>[4x]SAVKTNVGPSRAGVGYDVIVIGGGFAGVTAAREASRSGLKTLILEGRSRLGGRTFTSKLQNQKVELGGTWVHWTQPNVWTEIMHYGLEVEETVGLANPETVIWVTEDNVKRAPAAEAFEIFGSACNEYYKEARNIYPRPFEPFFERKKLQHVDGLSAADY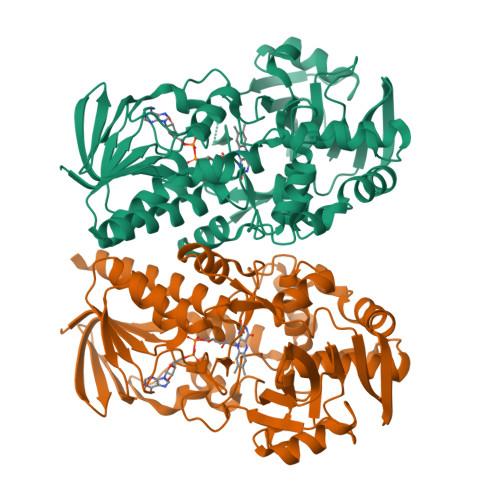LEKLPLTREQKDMMDSWLSGNGHNYPETIAYSEIMRWFALSNFNMPTMFDSIARYKIKTGTHSLLEAIMADGNSEVKLSTPVTKVNQDKDKVTVTTEDGVFTASAVIVAVPINTLHDIEYSPKLSAAKVDMGSQRHAGAGVKGYIRVKQNVGNVMTYAPARNKLTPFTSVFTDHVDESGTLLIAFSADPKLIDINDIKAVEKALQPLLPGVEVTASYGYDWNLDPFSKGTWCTYRPNQTTRYLTELQKREGRLFFAGSDMANGWRGFIDGAIENGREVGHQVATYLKRENDNA>[2x]MEYTQLGRIGLKVSRLVLGTMNFGPTTDEAESHAIMDAALDAGINFFDTANVYGWGENKGRTEEILGSWFAQGGDRRDKVVLATKVYGNMGLDGPAWPNHDKLSALNIRRSVDASLKRLGTDHIDLYQFHHVDRDTPWDEIWQAMDVLVRQGKILYVGSSNFAGWNIAQANETAARHGRLGLVSEQCLYNLCERRAEMEVVPAAREYGLGVIAWSPLHGGLLGGAIRKEQEGGNRRAASGRAADALKDPQQREQIQRYEDLLDKHGLEPGEVALAWLLTRPGVTGPIVGPRTADQLASAVRAAELTLTDEVLTALDEIFPGPGPSPEAFAW

Aldo-keto reductases (AKRs) are a superfamily of oxidoreductases capable of reducing carbonyl to primary and secondary alcohols, found in all phyla. In this work, we identify the enzyme AKRtyl, which is responsible for tylosin reduction. Phylogenetic analysis indicates that AKRtyl is the founding member of subfamily D within family 12 in the AKR superfamily. Specifically, by combining steady-state and transient kinetics, X-ray crystallography and molecular dynamics simulation, we demonstrate that AKRtyl exhibits a positive synergy mediated by an unusual Monod-Wyman-Changeux (MWC) paradigm of allosteric regulation at low concentrations of the cofactor NADPH, but an inhibitory effect at high concentrations is observed.

To obtain the apo structure of AKRtyl, we remove the carried cofactors by denaturation and refolding. We successfully obtained two apo structures of AKRtyl without any cofactor. The second apo structure has only two active conformational (R) subunits in an asymmetric unit, by combining with other asymmetric units, we can obtain an octamer containing two active tetramers (R4R4). We didn’t get the apo structures in the T4T4 state and speculate that structures in this state may not crystallize due to energetic issues. We therefore propose that the basic unit of MWC-type allosteric ensemble is a tetramer rather than an octamer for: (1) The tetramer exhibits ligand-independent T and R conformations, suggesting that the equilibrium between the T and R conformations occurs within the tetramer.>[6x]MRGSHHHHHHGSMEQSHQNLQSQFFIEHILQILPHRYPMLLVDRITELQANQKIVAYKNITFNEDVFNGHFPNKPIFPGVLIVEGMAQSGGFLAFTSLWGFDPEIAKTKIVYFMTIDKVK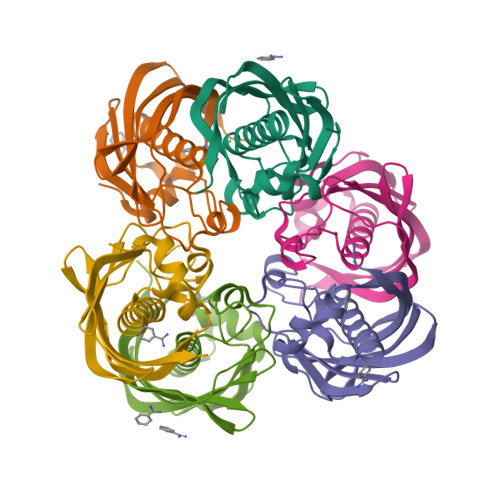FRIPVTPGDRLEYHLEVLKHKGMIWQVGGTAQVDGKVVAEAELKAMIAERE> MISTTISGKRPIEQVDDELLSLTAQQENEEQQQQRKRRRHQFAPMTQFNSNTLDEDSGFRSSSDVATADQDNFLEESPSGYIKKVILRNFMCHEHFELELGSRLNFIVGNNGSGKSAILTAITIGLGAKASETNRGSSLKDLIREGCYSAKIILHLDNSKYGAYQQGIFGNEIIVERIIKRDGPASFSLRSENGKEISNKKKDIQTVVDYFSVPVSNPMCFLSQDAARSFLTASTSQDKYSHFMKGTLLQEITENLLYASAIHDSAQENMALHLENLKSLKAEYEDAKKLLRELNQTSDLNERKMLLQA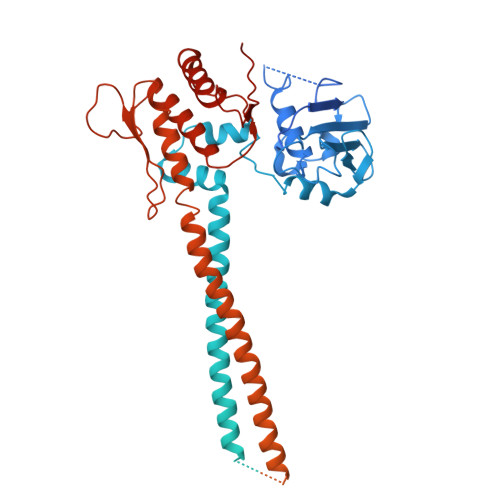KSLWIDVAHNTDACKNLENEISGIQQKVDEVTEKIRNRQEKIERYTSDGTTIEAQIDAKVIYVNEKDSEHQNARELLRDVKSRFEKEKSNQAEAQSNIDQGRKKVDALNKTIAHLEEELTKEMGGDKDQMRQELEQLEKANEKLREVNNSLVVSLQDVKNEERDIQHERESELRTISRSIQNKKVELQNIAKGNDTFLMNFDRNMDRLLRTIEQRKNEFETPAIGPLGSLVTIRKGFEKWTRSIQRAISSSLNAFVVSNPKDNRLFRDIMRSCGIRSNIPIVTYCLSQFDYSKGRAHGNYPTIVDALEFSKPEIECLFVDLSRIERIVLIEDKNEARNFLQRNPVNVNMALSLRDRRSGFQLSGGYRLDTVTYQDKIRLKVNSSSDNGTQYLKDLIEQETKELQNIRDRYEEKLSEVRSRLKEIDGRLKSTKNEMRKTNFRMTELKMNVGKVVDTGILNSKINERKNQEQAIASYEAAKEELGLKIEQIAQEAQPIKEQYDSTKLALVEAQDELQQLKEDINSRQSKIQKYKDDTIYYEDKKKVYLENIKKIEVNVAALKEGIQRQIQNACAFCSKERIENVDLPDTQEEIKRELDKVSRMIQKAEKSLGLSQEEVIALFEKCRNKYKEGQKKYMEIDEALNRLHNSLKARDQNYKNAEKGTCFDADMDFRASLKVRKFSGNLSFIKDTKSLEIYILTTNDEKARNVDTLSGGEKSFSQMALLLATWKPMRSRIIALDQFDVFMDQVNRKIGTTLIVKKLKDIARTQTIIITPQDIGKIADIDSSGVSIHRMRDPERQNNSNFYN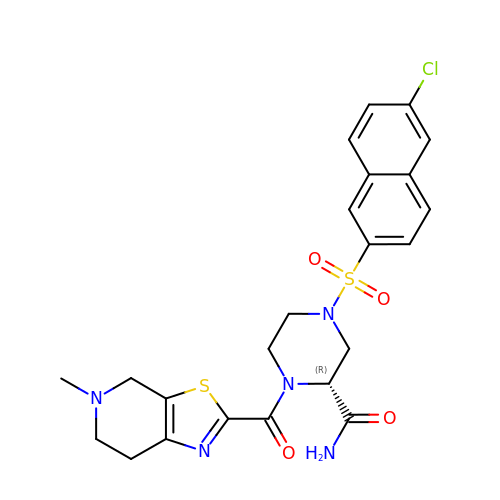(2R)-4-[(6-CHLORO-2-NAPHTHYL)SULFONYL]-1-[(5-METHYL-4,5,6,7-TETRAHYDRO[1,3]THIAZOLO[5,4-C]PYRIDIN-2-YL)CARBONYL]PIPERAZINE-2-CARBOXAMIDE | C23 H24 Cl N5 O4 S2 | OVHHNKPYYVQCLN-LJQANCHMSA-N> AQTVPYGIPLIKADKVQAQGFKGANVKVAVLDTGIQASHPDLNVVGGASFVAGEAYNTDGNGHGTHVAGTVAALDNTTGVLGVAPSVSLYAVKVLNSSGSGSYSGIVSGIEWATTNGMDVINMSLGGASGSTAMKQAVDNAYARGVVVVAAAGNSGNSGSTNTIGYPAKYDSVIA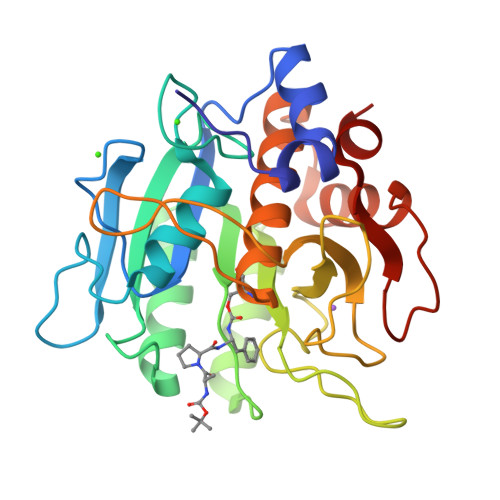VGAVDSNSNRASFSSVGAELEVMAPGAGVYSTYPTNTYATLNGTSMASPHVAGAAALILSKHPNLSASQVRNRLSSTATYLGSSFYYGKGLINVEAAAQAP> PTPCYISIEGQTQGLITAGACTADSIGDSFVEGHEDEMLVQQFDHVVTVPTDPQSGQPSGQRVHKPFKFTVALNKAVPLLYNALSSGEKLKTVELKWYRTSIEGKQENFFTTKLENASIVDIHCEMPHCQDPAKSDFTQNVTVSLSYRKITWDHVNAGTSGSDDW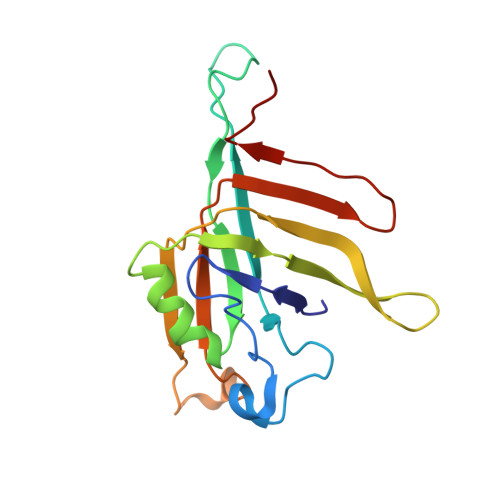RKPIE> MPTLLRVYIDGPHGMGKTTTTQLLVALGSRDDIVYVPEPMTYWRVLGASETIANIYTTQHRLDQGEISAGDAAVVMTSAQITMGMPYAVTDAVLAPHIGGEAGSSHAPPPALTLIFDRHPIAALLCYPAARYLMGSMTPQAVLAFVA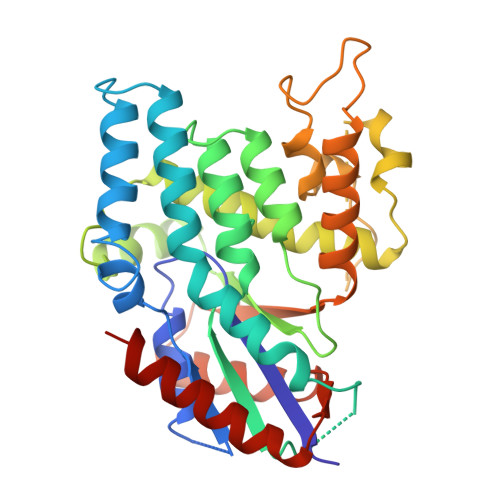LIPPTLPGTNIVLGALPEDRHIDRLAKRQRPGERLDLAMLAAIRRVYGLLANTVRYLQCGGSWREDWGQLSGTAVPPQGAEPQSNAGPRPHIGDTLFTLFRAPELLAPNGDLYNVFAWALDVLAKRLRSMHVFILDYDQSPAGCRDALLQLTSGMVQTHVTTPGSIPTICDLARTFAREMGEAN>GHMVSVAAGDKPTNSRQEILEGARRCFAEHGYEGATVRRLEEATGKSRGAIFHHFGDKENLFLALAREDAARMAEVVSENGLVEVMRGMLEDPERYDWMSVRLEISKQLRTDPVFRAKWIDHQSVLDEAVRVRLSRNVDKGQMRTDVPIEVLHTFLETVLDGFISRLATGASTEG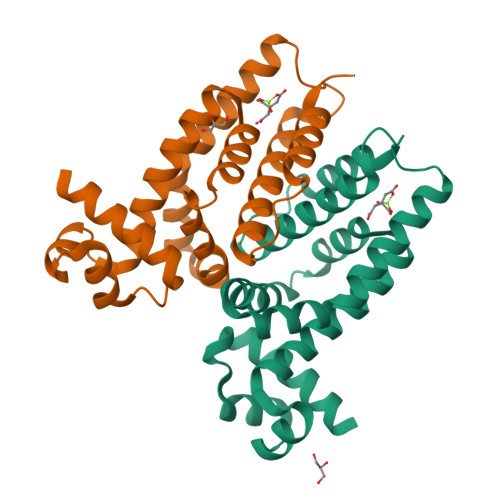LSEVLDLVEGTVRKRD[2x]> DPDIPENYDPRLIWPNCSSLFTIPDQANCGSCWAVSTAAAISDRLCIASKGENQVFISSADILSCCDTCGFGCDGGITFRAWEYFATKGSVSGGHFEAPNCCRPYYFHPCGQHGNDTFYGYCPRFAQTPFCRRKCRIGFNKSYAQDRIQGKSFYTVDYSVPAIQREIMTKGSVVGSYDVFTDFSHYKSGIYRHTGGKPDGRHAVRIIGWGKENGTDYWLIANSWHDDWG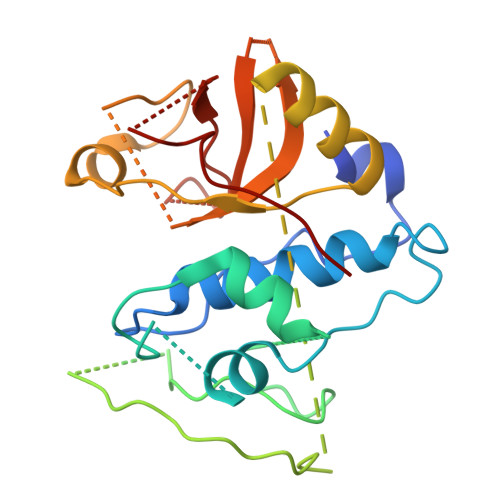ENGYFRMIRGINDCGIEQDITAGD[(1S)-3-methyl-1-[[(2S)-3-phenyl-2-(pyrazin-2-ylcarbonylamino)propanoyl]amino]butyl]boronic 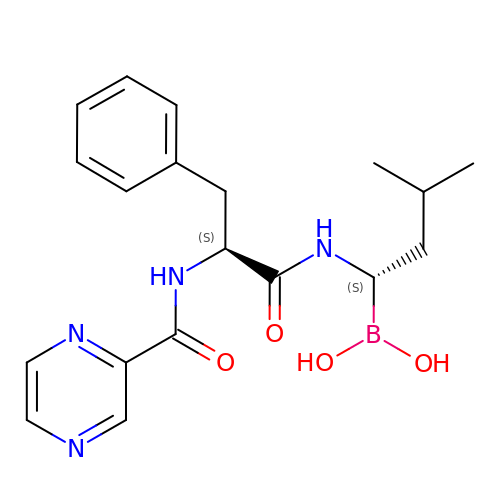acid | C19 H25 B N4 O4 | GXJABQQUPOEUTA-DOTOQJQBSA-N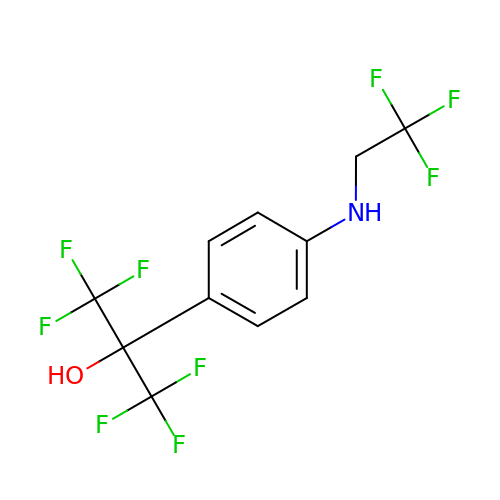1,1,1,3,3,3-HEXAFLUORO-2-{4-[(2,2,2-TRIFLUOROETHYL)AMINO]PHENYL}PROPAN-2-OL | C11 H8 F9 N O | VHDRSZOHKKZOQF-UHFFFAOYSA-N> FSQHARTSGRVAVEEVDEEGKFVRLRNKSNEDQSMGNWQIKRQNGDDPLLTYRFPPKFTLKAGQVVTIWAAGAGATHSPPTDLVWKAQNTWGCGNSLRTALINSTGEEVAMRKLVR;>TSQKHRDFVAEPMGEKPVGSLAGIGEVLGKKLEERGFDKAYVVLGQFLVLKKDEDLFREWLKDTAGANAKQSRDAFGALREWADAFL[2x];> DNYADLSDTELTTL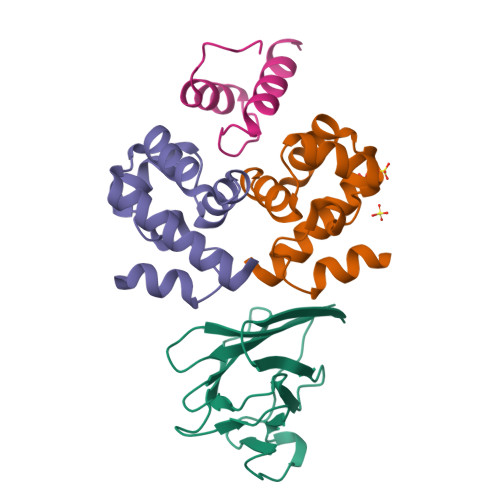LRRYNIPHGPVVGSTRRLYEKKIFEYEIQ> MHPFVKALQEHFTAHQNPEKAEPMARYMKNHFLFLGIQTPERRQLLKDIIQIHTLPDQKDFQIIIRELWDLPEREFQAAALDIMQKYKKHINETHIPFLEELIVTKSWWDSVDSIVPTFLGDIFLKHPELISAYIPKWIASDNIWLQRAAILFQLKYKQKMDEELLFWIIGQLHSSKEFFIQKAIGWVLREYAKTNPDVVWEYVQNNELAPLSKREAIKHIKQ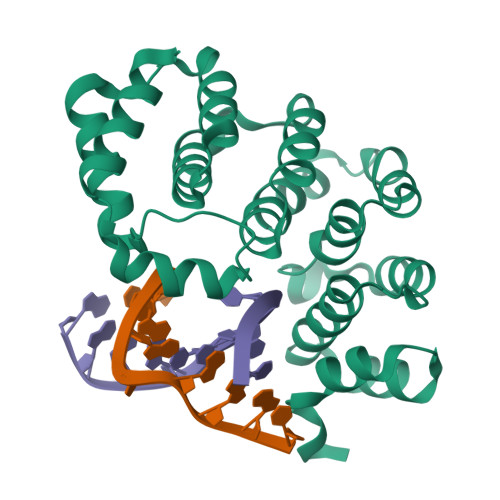NY> MAMANNSSVANKVCLIVIDGWGVSEDPYGNAILNAQTPVMDKLCSGNWAQIEAHGLHVGLPEGLMGNSEVGHLNIGAGRVIYQDIVRINLAVKNNKFVTNESLVDACDRAKNGNGRLHLAGLVSDGGVHSHIDHMFALVKAIKELGVPELYLHFYGDGRDTSPNSGVGFLEQTLEFLEKTTGYGKLATVVGRYYAMDRDNRWERINVAYEAMIGGVGETSDEAGVVEVVRKRYAADETDEFLKPIILQGEKGRVQNDDTIIFFDYRADRMREISAAMGMDRYKDCNSKLAHPSNLQVYGMTQYKAEFPFKSLFPPASNKNVLAEWLAEQKVSQFHCAETEKYAHVTFFFNGGLEKQFEGEERCLVPSPKVATYDLQPEMSAAGVADKMIEQLEAGTHPFIMCNFAPPDMVGHTGVYEAAVKACEATDIAIGRIYEATQKHGYSLMVTADHGNAEKMKAPDGGKHTAHTCYRVPLTLSHPGFKFVDPADRHPALCDVAPTVLAIMGL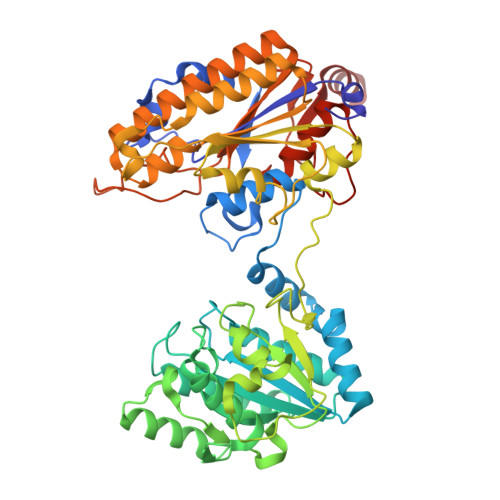PQPAEMTGVSIVQKIKLAAALEHHHHHH>[2x]SNGLEDSSTISFITWNIDGLDGCNLPERARGVCSCLALYSPDVVFLQEVIPPYCAYLKKRA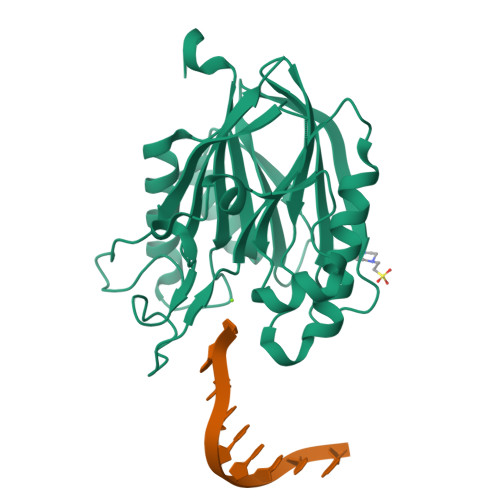ASYTIITGNEEGYFTAILLKKGRVKFKSQEIIPFPNTKMMRNLLCVNVSLGGNEFCLMTSHLESTREHSAERIRQLKTVLGKMQEAPDSTTVIFAGDTNLRDQEVIKCGGLPDNVFDAWEFLGKPKHCQYTWDTKANNNLRIPAAYKHRFDRIFFRAEEGHLIPQSLDLVGLEKLDCGRFPSDHWGLLCTLNVVL Mtb Decaprenylphosphoryl‐β‐d‐ribofuranose 2‐oxidase (DprE1) is a flavin adenine dinucleotide (FAD)‐dependent enzyme, which together with decaprenylphosphoryl‐d‐2‐ketoerythropentose reductase (DprE2), converts decaprenylphosphoryl‐beta‐d‐ribose (DPR) to decaprenylphosphoryl‐beta‐d‐arabinofuranose (DPA), an essential cell wall component. Multiple covalent3 and non‐covalent4 DprE1 inhibitors have been identified and showed in vitro and in vivo activities against Mtb, further validating DprE1 as an attractive anti‐tuberculosis (TB) drug target. When analyzing toxicity profiles, we noticed that many TCA1 analogs show inhibition of CYP2C9, one of six major cytochrome P450 enzymes which determine the clearance of 75 % of marketed drugs. Here we report the X‐ray crystal structures of WT DprE1, a TCA1‐resistant DprE1 mutant, and CYP2C9 in complex with TCA1 analogs.

KGaAThe thiophene ring is located in a hydrophobic pocket formed by Gly133, Lys367, Phe369 and Asn385 and accepts a H‐bond from His132 Nϵ2 (3.2 Å). Replacement of thiophene with other heterocycles or adding bulky substitutions resulted in reduced activity against Mtb (data not shown). Only a fluoro substituent on the thiophene afforded an analog (TCA481) that is 5‐fold more potent than TCA1 based on MIC. To better understand the basis of the activity increase, we solved the crystal structure of DprE1 in complex with TCA481. The structure reveals that the fluoro group forms a H‐bond with Asn385 Nδ2 (3.4 Å). The fluorine is accommodated in the pocket with stronger hydrophobic interactions with residues Phe369, His132, and Lys367 than TCA1.

>MGSSHHHHHHSQDPNSMLSVGATTTATRLTGWGRTAPSVANVLRTPDAEMIVKAVARVAESGGGRGAIARGLGRSYGDNAQNGGGLVIDMTPLNTIHSIDADTKLVDIDAGVNLDQLMKAALPFGLWVPVLPGTRQVTVGGAIACDIHGKNHHSAGSFGNHVRSMDLLTADGEIRHLTPTGEDAELFWATVGGNGLTGIIMRATIEMTPTSTAYFIADGDVTASLDETIALHSDGSEARYTYSSAWFDAISAPPKLGRAAVSRGRLATVEQLPAKLRSEPLKFDAPQLLTLPDVFPNGLANKYTFGPIGELWYRKSGTYRGKVQNLTQFYHPLDMFGEWNRAYGPAGFLQYQFVIPTEAVDEFKKIIGVIQASGHYSFLNVFKLFGPRNQAPLSFPIPGWNICVDFPIKDGLGKFVSELDRRVLEFGGRLYTAKDSRTTAETFHAMYPRVDEWISVRRKVDPLRVFASDMARRLELL[2x]>TDKLTSLRQYTTVVADTGDIAAMKLYQPQDATTNPSLILNAAQIPEYRKLIDDAVAWAKQQSNDRAQQIVDATDKLAVNIGLEILKLVPGRISTE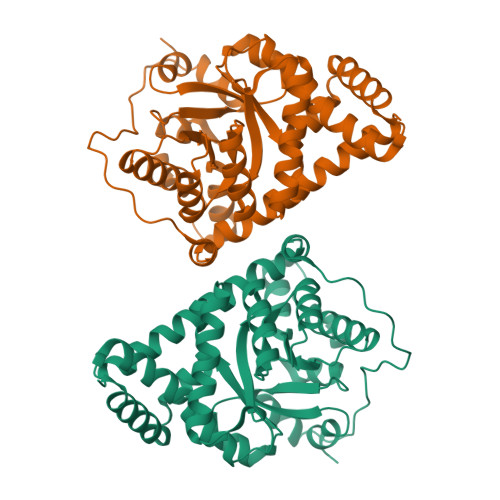VDARLSYDTEASIAKAKRLIKLYNDAGISNDRILIKLASTWQGIRAAEQLEKEGINCNLTLLFSFAQARACAEAGVFLIAPFVGRILDWYKANTDKKEYAPAEDPGVVSVSEIYQYYKEHGYETVVMGASFRNIGEILELAGCDRLTIAPALLKELAESEGAIERKLSYTGEVKARPARITESEFLWQHNQDPMAVDKLAEGIRKFAIDQEKLEKMIGDLL[2x]>NDEVPELRIEKVKENIFLHTSYSRVNGFGLVSSNGLVVIDKGNAFIVDTPWSDRDTETLVHWIRKNGYELLGSVSTHWHEDRTAGIKWLNDQSISTYATTSTNHLLKENKKEPAKYTLKGNESTLVDGLIEVFYPGGGHTIDNVVVWLPKSKILFGGCFVRSLDS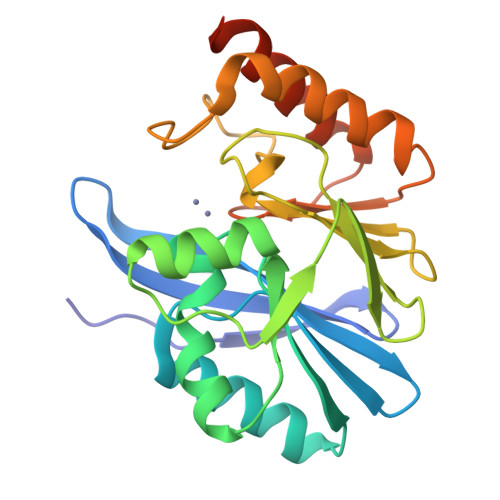EGLGYTGEAHIDQWSRSAQNALSRYSEAQIVIPGHGKIGDIALLKHTKSLAETASNKSIQPNANASAD[2x]>MTHHYPTDDIKIKEVKELLPPIAHLYELPISKEASGLVHRTRQEISDLVHGRDKRLLVIIGPCSIHDPKAALEYAERLLKLRKQYENELLIVMRVYFEKPRTT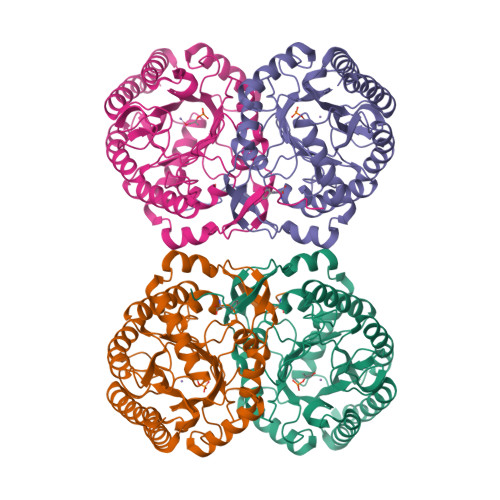VGWKGLINDPHLDGTFDINFGLRQARSLLLSLNNMGMPASTEFLDMITPQYYADLISWGAIGARTTESQVHRELASGLSCPVGFKNGTDGNLKIAIDAIGAASHSHHFLGVTKAGHSAIVHTGGNPDCHVILRGGKEPNYDAEHVSEAAEQLRAAGVTDKLMIDCSHANSRKDYTRQMEVAQDIAAQLEQDGGNIMGVMVESHLVEGRQDKPEVYGKSITDACIGWGATEELLALLAGANKKRMARAS[4x]> SIHTKLRKSSRGFGFTVVGGDEPDEFLQIKSLVLDGPAALDGKMETGDVIVSVNDTCVLGHTHAQVVKIFQSIPIGASVDLEL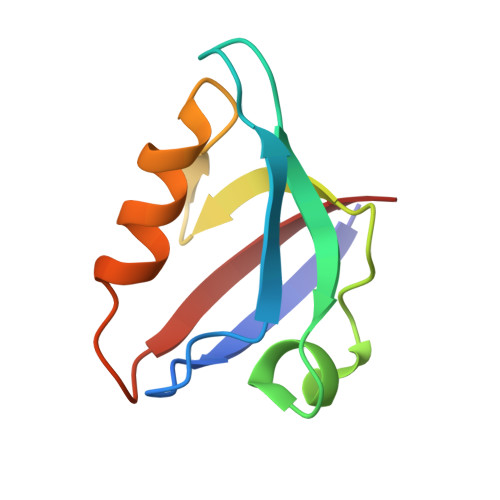CR>MHHHHHHENLYFQGGVSVQLEMKALWDEFNQLGTEMIVTKAGRRMFPTFQVKLFG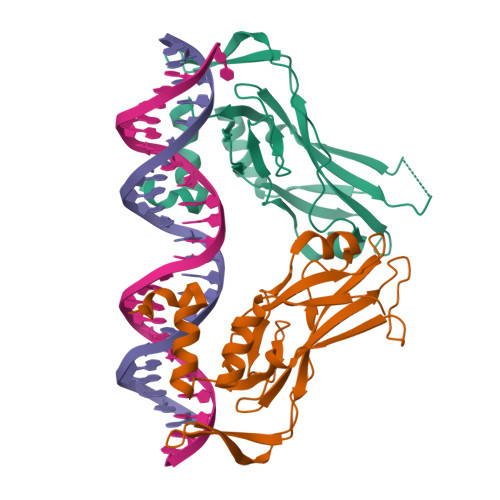MDPMADYMLLMDFVPVDDKRYRYAFHSSSWLVAGKADPATPGRVHYHPDSPAKGAQWMKQIVSFDKLKLTNNLLDDNGHIILNSMHRYQPRFHVVYVDPRKDSEKYAEENFKTFVFEETRFTAVTAYQNHRITQLKIASNPFAKGFRD[2x]>AQVINTFDGVADYLQTYHKLPDNYITKSEAQALGWVASKGNLADVAPGKSIG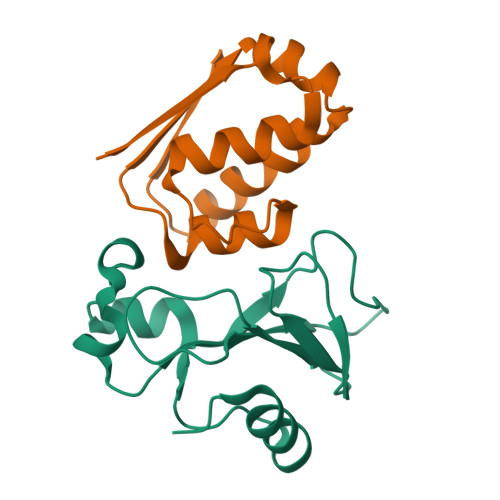GDIFSNREGKLPGKSGRTWREADINYTSGFRNSDRILYSSDWLIYKTTDHYQTFTKIR[3x];>MKKAVINGEQIRSISDLHQTLKKELALPEYYGENLDALWDALTGWVEYPLVLEWRQFEQSKQLTENGAESVLQVFREAKAAGADITIILS[3x]> QAQITGRPEWIWLALGTALMGLGTLYFLVKGMGVSDPDAKKFYAITTLVPAIAFTMYLSMLLGYGLTMVPFGGEQNPIYWARYADWLFTTPLLLLDLALLVDADQGTILALVGADGIMIGTGLVGALTKVYSYRFVWWAISTAAMLYILYVLFFGFTSKAESMR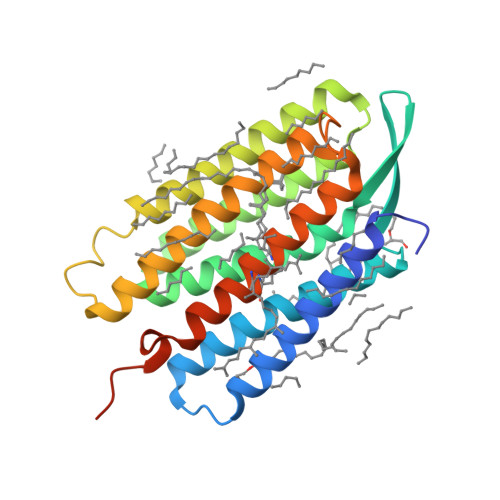PEVASTFKVLRNVTVVLWSAYPVVWLIGSEGAGIVPLNIETLLFMVLDVSAKVGFGLILLRSRAIFGEAEAPEPSAGDGAAATS>[4x]MIISKEKTVSQEEMEELRLVARKTWRYFEDFVTEGQNYLPPDNFQEDPPNGVAERTSPTNIGLYLVSVIGARDLGYITTTEMVERIKKTLDTIEKMEKWNGHLYNWYNTKTLEPLRPYYVSTVDSGNLVGYLITVKEAIGEFLNKPLIDIELAKGLKDTIKMLNVKGITEDIFTTILSKTTLVPSEWEAFLNKIREKLLSSQDDLENIKRLKNIIIALKGEMKEFLVWTEFDESEKEQEIFKRYKEVFEEHSSPKELEKVYKNYLLEIEEVFKKATEEEKALLKSQKDKVAQALEKIKKLEAEIENIKSTIENLVEKTEFRHLYDEKRQLFSIGYNVEEEKLTKSYYD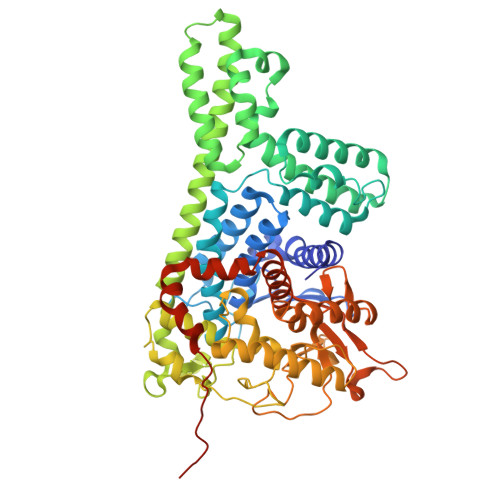LLASEARQASFIAIAKKEVDKKHWFKLGRMLAIENRYKGLVSWSGTMFEYFMPLLVMRNYQNTLLDETYAFAVRVQKNYAKELGIPWGISESGFYAFDMNLNYQYKAFGVPSLGLKRGLSHDKVVAPYGSLLAIGVDVEGVLQNIRFFKKEGAEGKYGFYEAIDYTPERVPFGKKSAIVKSFMAHHQGMVFVALDNFINNNVMQKRFHKDPRIKAAQILLQEKMPMYLDITREEREGARKLEHHHHHH> MHHHHHHMGIVTGPIIDHSKENDVMNEAEQNAETVRRGYAAFNSGDMKTLTELFDENASWHTPGRSRIAGDHKGREAIFAQFGRYGGETGGTFKAVLLHVLKSDDGRVIGIHRNTAERGGKRLDVGCCIVFEFKNGRVID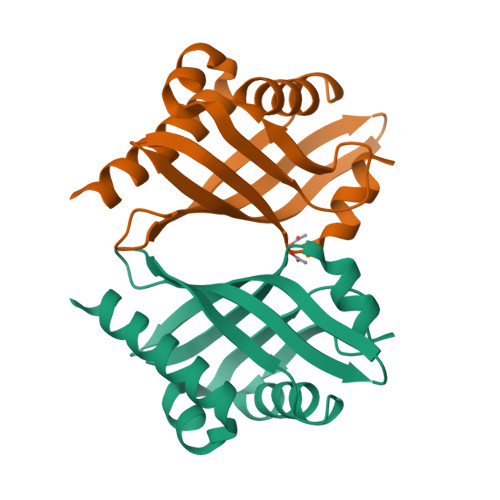GREHFYDLYAWDEFWR> ADLTASTTRTATLVEPARITLTYKEGAPITIMDNGNIDTELLVGTLTLGGYKTGT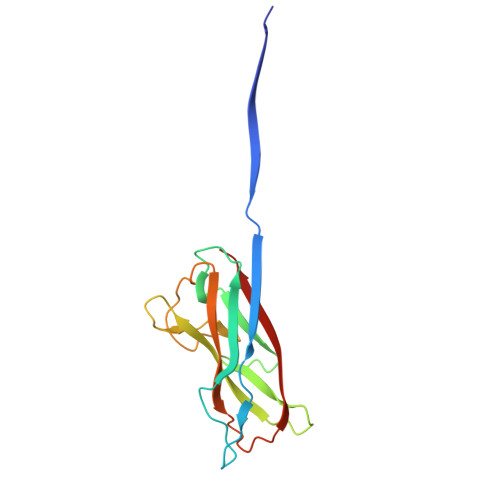TSTSVNFTDAAGDPMYLTFTSQDGNNHQFTTKVIGKDSRDFDISPKVNGENLVGDDVVLATGSQDFFVRSIGSKGGKLAAGKYTDAVTVTVSNQ>[2x]MRKLKYNTTRVILMIAFISLSACSSEDAMIEEEQVIPDPDPVAQTDEDTGPVVDCTNQGTNPTRDTDIPNPRNIGDIDDRSCYANYSESSILGKFWGIYNITDGSNHMDAP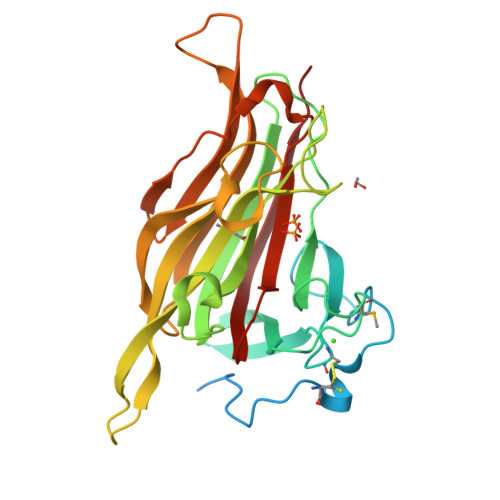NTLQPRIERSLSRSQATGAGSYARFRGVLRILEVGDTGTFSSSGSYFMQAKGKHTGGGGSPDPAICLYRAHPVYGDDGNGNQVQVSFDIWREQINFRGGSGSAGRTEVFLKNVLKNEQIDIELEVGFRDDPNNPGQTLHYADAKIGGEEFNWNIPEPERGIESGIRYGAYRVKGGRAQFRWANTSYTKDEVN> MGSDKIHHHHHHMVRVRFAPSPTGFLHVGGARTALFNFLFARKEKGKFILRIEDTDLERSEREYEEK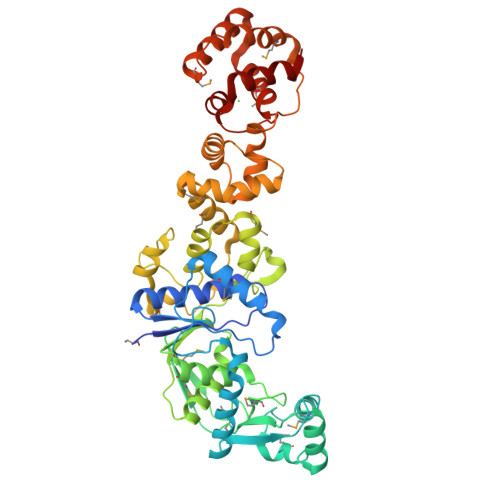LMESLRWLGLLWDEGPDVGGDHGPYRQSERVEIYREHAERLVKEGKAYYVYAYPEEIEEMREKLLSEGKAPHYSQEMFEKFDTPERRREYEEKGLRPAVFFKMPRKDYVLNDVVKGEVVFKTGAIGDFVIMRSNGLPTYNFACVVDDMLMEITHVIRGDDHLSNTLRQLALYEAFEKAPPVFAHVSTILGPDGKKLSKRHGATSVEAFRDMGYLPEALVNYLALLGWSHPEGKELLTLEELISSFSLDRLSPNPAIFDPQKLKWMNGYYLRNMPIEKLAELAKPFFEKAGIKIIDEEYFKKVLEITKERVEVLSEFPEESRFFFEDPAPVEIPEEMKEVFSQLKEELQNVRWTMEEITPVFKKVLKQHGVKPKEFYMTLRRVLTGREEGPELVNIIPLLGKEIFLRRIERSLGG> MHHHHHHMITVDKRPSSRGYDDWRLSDIPQYKDGISTYEFVRATHEADYRTHQAEPVAGRTFGFNGIGRLTEVALHMPTRYTLHDQSSQYKESPSFFQGLMGVPDRGPVDLAAFQRETEELATAFENNGIKVHWVDYPEEPANPYGPLMGHVFLSWGSIWRGGSVISRFGFLPGMVGVSEYLAKWAWNTLNIPPLVAITEGAMEPGACNMIADEVLVTCLSASYDQRGTDQLVAAISKTSGTEEFHNLQLRPAVEGFFNKATGACAHPDININAIDVGKLVVSPAALDWDARTWLYDNNFELIEADPDEQREFLAPCNVLLLEPGKVIAHADCHKTNQKIRDAGVEVIEVTGTEIRKACGGIKARVMQINREPGPTLADVRNRVWR

Mycobacterium sp. JS330 produces 2-nitroimidazole nitrohydrolase (NnhA) that circumvents 2NI activation, conferring 2NI resistance by hydrolysing it to nitrite and imidazol-2-one (IM2O) instead. The initial characterization of NnhA indicated that, unlike most other known enzymes that degrade nitroaromatic compounds, NnhA is a hydrolase that functions without catalytic metal ions, molecular oxygen, or other cofactors. Despite low sequence similarity and limited occurrence in a few soil-dwelling mycobacteria and Actinomycetota, NnhA maintains the α/β propeller fold characteristic of GME superfamily enzymes and forms an unusual hexameric ring structure formed by a trimer of domain-swapped dimers. The residues in the active site of NnhA appear somewhat conserved in comparison to the ADI and DDAH, with the catalytic histidine, glutamic acid, and cysteine residues present in NnhA as H260, E197, and C357.

We also crystallized and solved the structure of an active site variant NnhA-T2I-G14D-K73R-C357A, in which the presumptive nucleophilic cysteine residue had been substituted for an alanine residue. To investigate which of these cysteine residues is likely to be the catalytic nucleophile for the reaction, we substituted either C352 or C357 for either alanine or serine residues in addition to the T2I, G14D, and K73R mutations. We found that despite soluble expression, C357A and C357S substitutions eliminated activity. On the other hand, the C352A variant still retained activity with fivefold lower catalytic efficiency than the base NnhA-T2I-G14D-K73R variant, and the C352S variant also retained detectable activity despite its poor soluble expression that prevented protein purification for detailed enzyme kinetics. This suggests that of these two cysteine residues, C357 is more likely to be the nucleophile in NnhA, fulfilling a similar role to the nucleophilic cysteine in ADI and DDAH that are conserved in the same structural position. The two catalytic mutant NnhA C357A structures solved in the H32 space group also adopt the same hexameric structure. To better understand the reaction mechanism of 2NI hydrolysis by NnhA, we tried to co-crystallize and soak 2NI into both the active and inactive (C357A) soluble NnhA crystals. However, no excess density for the 2NI moiety could be found in any of these structures. The only notable difference between the apo structures of the two variants was in the conformation of D262 at the active site. While D262 exists in two rotomeric conformations in soluble NnhA, only one conformation with a slight displacement is seen in the structure of the C357A mutant of soluble NnhA. Hence, it is possible that D262 has mobility within the active site, which may play a role in the catalytic mechanism.2-[[(2~{R},3~{S},4~{R},5~{R})-5-(6-aminopurin-9-yl)-3,4-bis(oxidanyl)oxolan-2-yl]methyl-[3-[6-azanyl-9-[(2~{R},3~{R},4~{S},5~{R})-5-[(3-azanylpropylcarbamoylamino)methyl]-3,4-bis(oxidanyl)oxolan-2-yl]purin-8-yl]prop-2-ynyl]amino]ethanoic acid | C29 H38 N14 O9 | 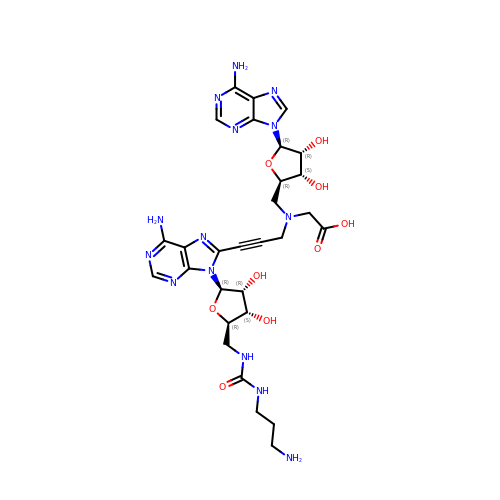PFWXIFMXYVCTQE-CGZJSAOLSA-N(2E)-5-[(diaminomethylidene)amino]-2-iminopentanoic 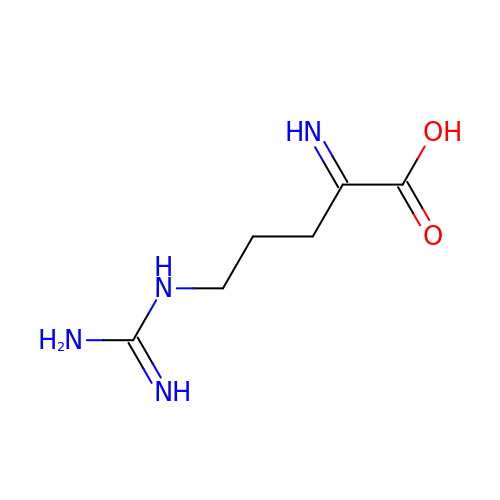acid | C6 H12 N4 O2 | YWGYOCPWFDUKSA-QPJJXVBHSA-N> GPGDQRFGDLVFRQLAPNVWQHTSYLDMPGFGAVASNGLIVRDGGRVLVVDTAWTDDQTAQIL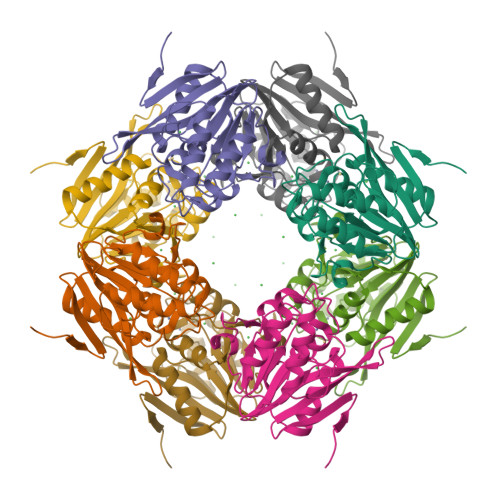NWIKQEINLPVALAVVTHAHQDKMGGMDALHAAGIATYANALSNQLAPQEGMVAAQHSLTFAANGWVEPATAPNFGPLKVFYPGPGHTSDNITVGIDGTDIAFGGCLIKDSKAKSLGNLGDADTEHYAASVRAFGAAFPKASMIVMSHSAPDSRAAITHTARMADKLR>[2x]QSMKIADIETFANEFVCFVKVTTDSGETGWGQVAPYYADITAQVLHRQVAPYALGKPALDIDYLVDIIPEKEHKFPGSYLRRALGGLDTALWDLRGRLEGKPVCELIGGTPGTVRAYGSSMKRDITPKDEAARLSRLRDRFGFDAFKFRIGAEC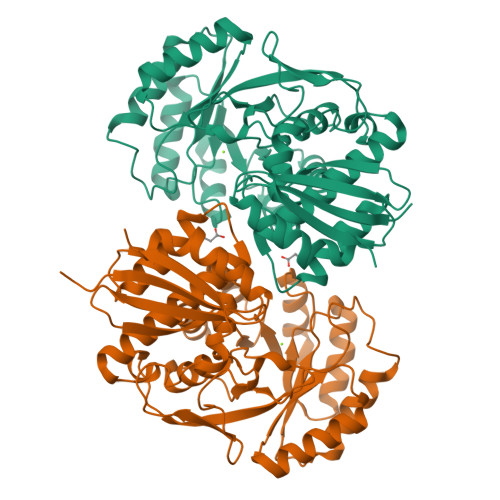GRGQDEWPGRTEEIVPTIRAAMDDSVALLVDANSCYGPEQAIEVGKMLEQNGISHYEEPCPYWEYEQTQQVTNALSIDVTGGEQDCELQNWRRMIEMKAVDIVQPDICYLGGITRTLRVAEMAHKAGLPCTPHAANLSMVTLFTMHLLRAIPNAGKYLEFSIEGEDYYPWQDDLFVASPYEIVDGKATVTDLPGWGVEVSPTWLETSAHQISTWQR> GPVLEATMICIDNSEWMRNGDYSPSRLQAQTEAVNLLCGAKTQSNPENTVGILTMAGKGVRVLTTPTSDLGKILA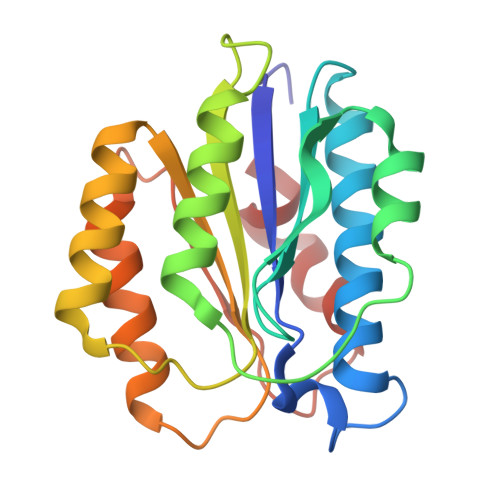CMHGLDVGGEINLTAAIQIAQLALKHRQNKNQRQRIIVFAGSPIKYEKKALEIVGKRLKKNSVSLDIVNFGEDDDEEKPQKLEALLTAVNNNDGSHIVHVPSGANALSDVLLSTPVFTG>[3x]MEKSLVDTVYALKDEVQELRQDNKKMKKSLEEEQRARKDLEKLVRKVLKNMNDPAWDETNL;> MGSSHHHHHHSQDPLVPRGSGSDYIIKEKTV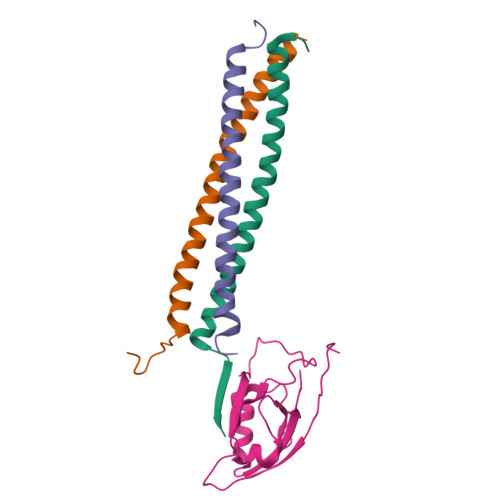LLQKKDSEGFGFVLRGAKAQTPIEEFTPTPAFPALQYLESVDEGGVAWRAGLRMGDFLIEVNGQNVVKVGHRQVVNMIRQGGNTLMVKVVMVTRHPDMDEA>[4x]ARFEEQKLYIGGRYVEASSGATFETINPANGEVLAKVQRASREDVERAVQSAVEGQKVWAAMTAMQRSRILRRAVDILRERNDELAALETLDTGKPLAETRSVDIVTGADVLEYYAGLVPAIEGEQIPLRETSFVYTRREPLGVVAGIGAWNYPVQIALWKSAPALAAGNAMIFKPSEVTPLTALKLAEIYTEAGVPDGVFNVLTGSGR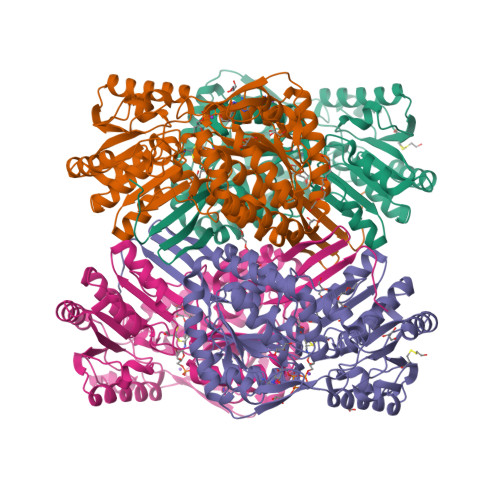EVGQWLTEHPLIEKISFTGGTSTGKKVMASASSSSLKEVTMELGGKSPLIIFPDADLDRAADIAVMANFFSSGQVCTNGTRVFIHRSQQARFEAKVLERVQRIRLGDPQDENTNFGPLVSFPHMESVLGYIESGKAQKARLLCGGERVTDGAFGKGAYVAPTVFTDCRDDMTIVREEIFGPVMSILVYDDEDEAIRRANDTEYGLAAGVVTQDLARAHRAIHRLEAGICWINTWGESPAEMPVGGYKQSGVGRENGLTTLAHYTRIKSVQVELGDYASVF>MRLKELGEFGLIDLIKKTLESKVIGDDTAPVEYCSKKLLLTTDVLNEGVHFLRSYIPEAVGWKAISVNVSDVIANGGLPKWALISLNLPEDLEVSYVERFYIGVKRACEFYKCEVVGGNISKSEKIGISVFLVGETER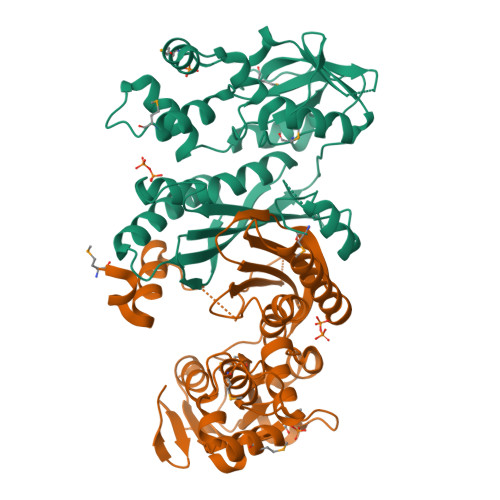FVGRDGARLGDSVFVSGTLGDSRAGLELLLMEKEEYEPFELALIQRHLRPTARIDYVKHIQKYANASMDISDGLVADANHLAQRSGVKIEILSEKLPLSNELKMYCEKYGKNPIEYALFGGEDYQLLFTHPKERWNPFLDMTEIGRVEEGEGVFVDGKKVEPKGWKHF[2x]> MDSTSTIANKIEEYLGAKSDDSKIDELLKADPSEVEYYRSGGDGDYLKNNICKITVNHSDSGKYDPCEKKLPPYDDNDQWKCQQNSSDGSGKPENICVPPRRERLCTYNLENLKFDKIRDNNAFLADVLLTARNEGEKIVQNHPDTNSSNVCNALERSFADLADIIRGTDQWKGTNSNLEKNLKQMFAKIRENDKVLQDKYPKDQKYTKLREAWWNANRQKVWEVITCGARSNDLLIKRGWRTSGKSDRKKNFELCRKCGHYEKEVPTKLDYVPQFLRWLTEWIEDFYREKQNLIDDMERHREECTREDHKSKEGTSYCSTCKDKCKKYCECVKKWKTEWENQENKYKDLYEQNKNKTSQKNTSRYDDYVKDFFEKLEANYSSLENYIKGDPYFAEYATKLSFILNPSDANNPSGETANHNDEACNCNESGISSVGQAQTSGPSSNKTCITHSSIKTNKKKECKDVKLGVRENDKDLKICVIEDTSLSGVDNCCCQDLLGILQENCSDNKRGSSSNDSCDNKNQDECQKKLEKVFASLTNGYKCDKCKSGTSRSKKKWIWKKSSGNEEGLQEEYANTIGLPPRTQSLYLGNLPKLENVCEDVKDINFDTKEKFLAGCLIVSFHEGKNLKKRYPQNKNSGNKENLCKALEYSFADYGDLIKGTSIWDNEYTKDLELNLQNNFGKLFGKYIKKNNTAEQDTSYSSLDELRESWWNTNKKYIWTAMKHGAEMNITTCNADGSVTGSGSSCDDIPTIDLIPQYLRFLQEWVENFCEQRQAKVKDVITNCKSCKESGNKCKTECKTKCKDECEKYKKFIEACGTAGGGIGTAGSPWSKRWDQIYKRYSKHIEDAKRNRKAGTKNCGTSSTTNAAASTDENKCVQSDIDSFFKHLIDIGLTTPSSYLSNVLDDNICGADKAPWTTYTTYTTTEKCNKERDKSKSQSSDTLVVVNVPSPLGNTPYRYKYACQCKIPTNEETCDDRKEYMNQWSCGSARTMKRGYKNDNYELCKYNGVDVKPTTVRSNSSKLDGNDVTFFNLFEQWNKEIQYQIEQYMTNANISCIDEKEVLDSVSDEGTPKVRGGYEDGRNNNTDQGTNCKEKCKCYKLWIEKINDQWGKQKDNYNKFRSKQIYDANKGSQNKKVVSLSNFLFFSCWEEYIQKYFNGDWSKIKNIGSDTFEFLIKKCGNNSAHGEEIFSEKLKNAEKKCKENESTDTNINKSETSCDLNATNYIRGCQSKTYDGKIFPGKGGEKQWICKDTIIHGDTNGACIPPRTQNLCVGELWDKSYGGRSNIKNDTKELLKEKIKNAIHKETELLYEYHDTGTAIISKNDKKGQKGKNDPNGLPKGFCHAVQRSFIDYKNMILGTSVNIYEHIGKLQEDIKKIIEKGTPQQKDKIGGVGSSTENVNAWWKGIEREMWDAVRCAITKINKKNNNSIFNGDECGVSPPTGNDEDQSVSWFKEWGEQFCIERLRYEQNIREACTINGKNEKKCINSKSGQGDKIQGACKRKCEKYKKYISEKKQEWDKQKTKYENKYVGKSASDLLKENYPECISANFDFIFNDNIEYKTYYPYGDYSSICSCEQVKYYKYNNAEKKNNKSLCYEKDNDMTWSKKYIKKLENGRSLEGVYVPPRRQQLCLYELFPIIIKNEEGMEKAKEELLE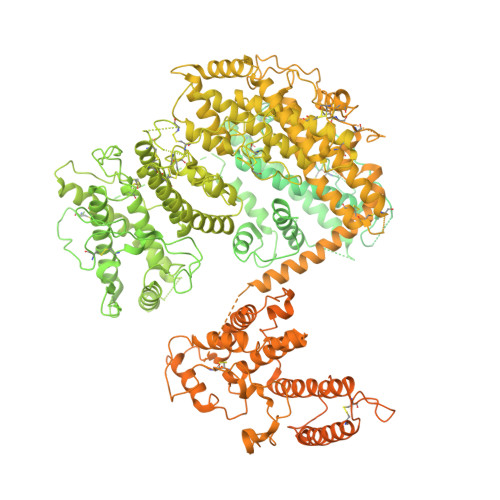TLQIVAEREAYYLWKQYNPTGKGIDDANKKACCAIRGSFYDLEDIIKGNDLVHDEYTKYIDSKLNEIFGSSNTNDIDTKRARTDWWENETITNGTDRKTIRQLVWDAMQSGVRYAVEEKNENFPLCMGVEHIGIAKPQFIRWLEEWTNEFCEKYTKYFEDMKSKCDPPKRADTCGDNSNIECKKACANYTNWLNPKRIEWNGMSNYYNKIYRKSNKESEDGKDYSMIMAPTVIDYLNKRCHGEINGNYICCSCKNIGAYNTTSGTVNKKLQKKETECEEEKGPLDLMNEVLNKMDKKYSAHKMKCTEVYLEHVEEQLNEIDNAIKDYKLYPLDRCFDDQTKMKVCDLIADAIGCKDKTKLDELDEWNDMDLRGTYNKHKGVLIPPRRRQLCFSRIVRGPANLRSLNEFKEEILKGAQSEGKFLGNYYKEHKDKEKALEAMKNSFYDYEDIIKGTDMLTNIEFKDIKIKLDRLLEKETNNTKKAEDWWKTNKKSIWNAMLCGYKKSGNKIIDPSWCTIPTTETPPQFLRWIKEWGTNVCIQKQEHKEYVKSKCSNVTNLGAQASESNNCTSEIKKYQEWSRKRSIQWETISKRYKKYKRMDILKDVKEPDANTYLREHCSKCPCGFNDMEEMNNNEDNEKEAFKQIKEQVKIPAELEDVIYRIKHHEYDKGNDYICNKYKNIHDRMKKNNGNFVTDNFVKKSWEISNGVLIPPRRKNLFLYIDPSKICEYKKDPKLFKDFIYWSAFTEVERLKKAYGGARAKVVHAMKYSFTDIGSIIKGDDMMEKNSSDKIGKILGDTDGQNEKRKKWWDMNKYHIWESMLCGYREAEGDTETNENCRFPDIESVPQFLRWFQEWSENFCDRRQKLYDKLNSECISAECTNGSVDNSKCTHACVNYKNYILTKKTEYEIQTNKYDNEFKNKNSNDKDAPDYLKEKCNDNKCECLNKHIDDKNKTWKNPYETLEDTFKSKCDCPKPLPSPIKPDDLPPQADEPFLESRGPFEGKPIPNPLLGLDSTRTGHHHHHH>[5x]MVKYQYEFPLDKAGKAGAVKPYRGGKNDFVTPVSNLSGVAEILTNAALKATEAYSQLGQDRLGAVLISKVKGWAYADREGTLFIEESDNNNVWTTTAAVNVAAGVLTATDWVYLSKRYYRFRYVNGNLQQSEFVLYQSVGAGEMDVRVNEKTPLQIDFAENQTHDGRLKVEARKTFDFVFHENAESASEGAALPVDGAAHLLVEVYGTAEMSEVKFWGKSV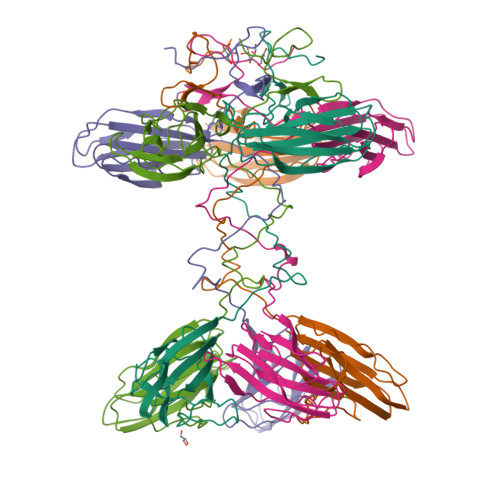SGQKLPIRGVKTDDATTASSTLGKAEAWAFDIKGFKEIIMEIISITGGTLSVKGTAVS2-amino-2-deoxy-6-O-sulfo-alpha-D-glucopyranose | C6 H13 N O8 S | 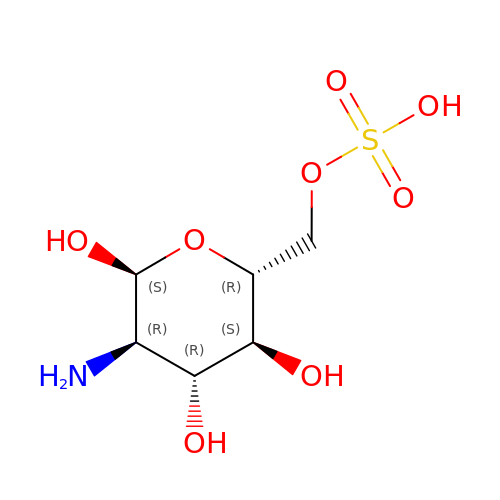MTDHILKWIRSIHB-UKFBFLRUSA-N>SNADASQFPQLTKEVGKEEAKVVMRTSQGDITLKLFPKYAPLAVENFLTHAKKGYYDNLTFHRVINDFMIQSGDPKGDGTGGESIWKGKDPKKDAGNGFVNEISPFLYHIRGALA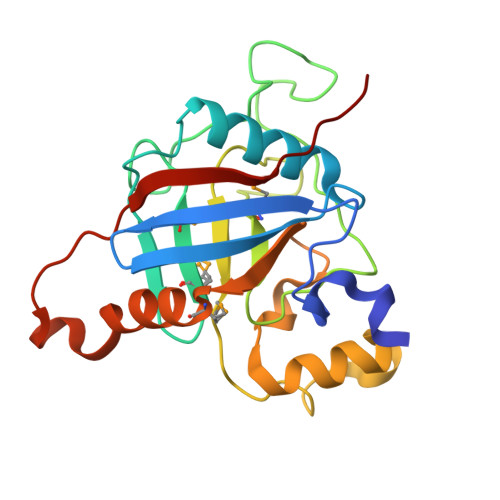MANAGANTNGSQFYINQNKKNQSKGLSSTNYPKPIISAYEHGGNPSLDGGYTVFGQVIDGMDVVDKIAATSINQNDKPEQDITITSIDIVKDYRFKN[2x]N-[(2S)-1-(azetidin-1-yl)propan-2-yl]-3-{2-[(3,5-dimethoxyphenyl)amino]pyrimidin-4-yl}-1-methyl-1H-pyrazole-5-carboxamide | C23 H29 N7 O3 | 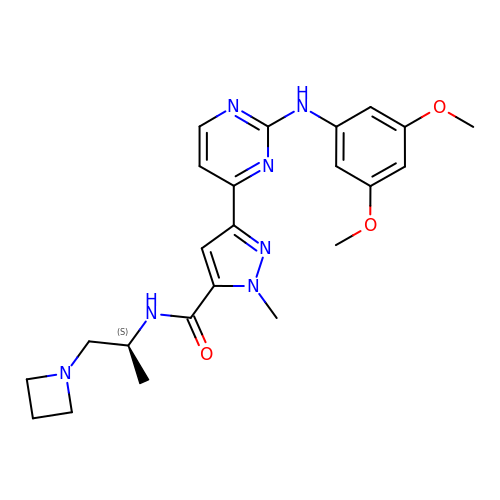YLCFOHVAOBLAIK-HNNXBMFYSA-N The universal stress proteins (USP) family member UspE is a tandem-type USP that consists of two Usp domains. The UspE expression levels of the Escherichia coli (E. coli) become elevated in response to oxidative stress and DNA damaging agents, including exposure to mitomycin C, cadmium, and hydrogen peroxide. UspA, UspC, and UspD belong to class I; UspF and UspG belong to class II; two Usp domains of UspE belong to class II and IV based on the sequence and structural analysis. USPs might be associated with several functions, such as cadmium binding, ATPase activity, and an intermediate in lipid A biosynthesis.

Specifically, it presents the three-dimensional X-ray crystal structure of the recombinantly produced UspE from E. coli at 3.2 Å resolution. UspE exists as a monomer, and the structure reveals a compact and 2-fold symmetric dimer in the crystal. The crystal structure shows that UspE is folded into a fan-shaped structure similar to that of the tandem-type Usp protein USP from P. mirabilis. UspE is composed of ten β-stranded mixed β-sheet and nine α-helices. More importantly, we found an unambiguous stick-like electron density in the hydrophobic pocket of E. coli UspE throughout the refinement process. In addition, the stick-like electron densities were very similar to a 3-hydroxymyristoyl group of Uridine-5′-diphosphate-3-O-(R-3-hydroxymyristoyl)-N-acetyl-D-glucosamine. The characteristic hydrophobic environment in the pocket indicates that UspE can bind unidentified ligand with a 3-hydroxymyristoyl group in the cavity. This pocket was surrounded by hydrophobic residues in β6, β9, β10, and α6. However, the ATP binding motif of UspE was disordered in the crystal, due to the intrinsic flexibility of these regions. Our structural analysis indicates that E. coli has two putative binding sites (Site I: His117, His 119; Site II: His193, His244).

>MAMYQNMLVVIDPNQDDQPALRRAVYLHQRIGGKIKAFLPIYDFSYEMTTLLSPDERTAMRQGVISQRTAWIHEQAKYYLNAGVPIEIKVVWHNRPFEAIIQEVISGGHDLVLKMAHQHDRLEAVIFTPTDWHLLRKCPSPVWMVKDQPWPEGGKALVAVNLASEEPYHNALNEKLVKETIELAEQVNHTEVHLVGAYPVTPINIAIELPEFDPSVYNDAIRGQHLLAMKALRQKFGINENMTHVEKGLPEEVIPDLAEHLQAGIVVLGTVGRTGISAAFLGNTAEQVIDHLRCDLLVIKPDQYQTPVELDDEEDD[2x]>MATTASAQKVGKATNKISGGDNNTANGTYLTIGGGDYNKTKGRYSTIGGGLFNEATNEYSTIGSGGYNKAKGRYSTIGGGGYNEATNQYSTIGGGDNNTAKGRYSTIGGGGYNEATIENSTVGGGGYNQAKGRNSTVAGGYNNEATGTDSTIAGGRKNQATGKGSFAAGIDNKANADNAVALGNKNTIEGENSVAIGSNNTVKKGQQNVFILGSNTDTTNAQNGSVLLGHNTAGKAATIVNSAEVGGLSLTGFAGASKTGNGTVSVGKKGKERQ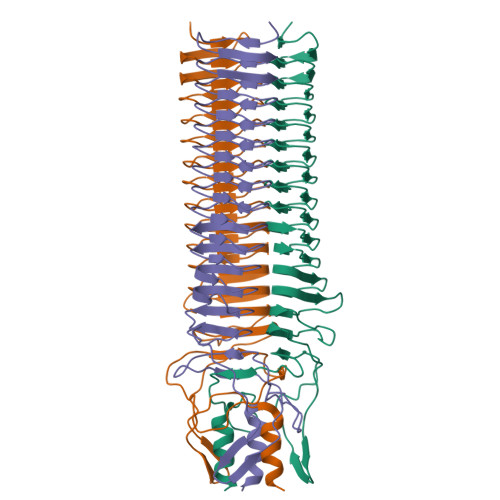IVHVGAGEISDTSTDAVNGSQLHALATVVAKHHHHHH[3x]(1~{Z},3~{E},5~{R},8~{S})-2,8-dimethyl-5-propan-2-yl-cyclodeca-1,3-diene 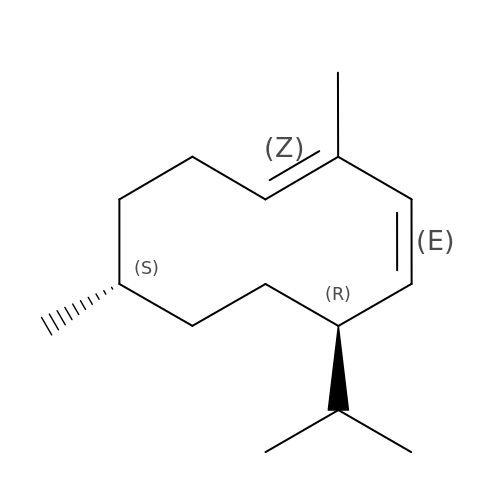| C15 H26 | KLGULIQQGMAJOK-XPXAULBRSA-N deltarasin | C40 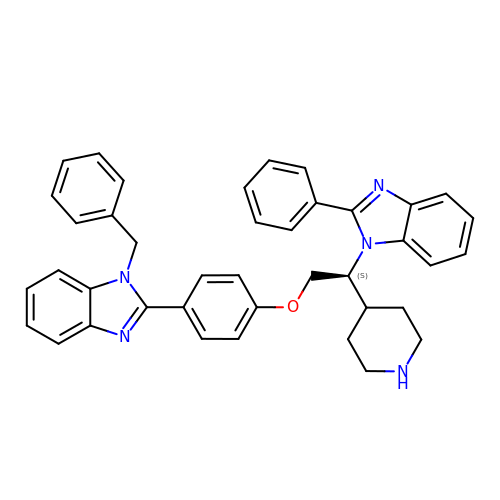H37 N5 O | LTZKEDSUXKTTTC-KXQOOQHDSA-N> GASDSPMAYTDGSYQFILNADNTATITKYTGNEHRITIPAQVTHGAYIYPVSKIGDRVFCNYKYVLTSVQIPDTVTEIGSNAFYNCTSLKRVTIQDNKPSCVKKIGRQAFMFCSELTDIPILDSVTEIDSEAFHHCEELDTVTIPEGVTSVADGMFSYCYSLHTVTLPDSVTAIEERAFTGTALTQIHIPAKVTRIGTNAFSECFALSTITSDSESYPAIDNVLYEKSANGDYALIRYPSQREDPAFKIPNGVARIETHAFDSCAYLASVKMPDSVVSIGTGAFMNCPALQDIEFSSRITELPESVFAGCISL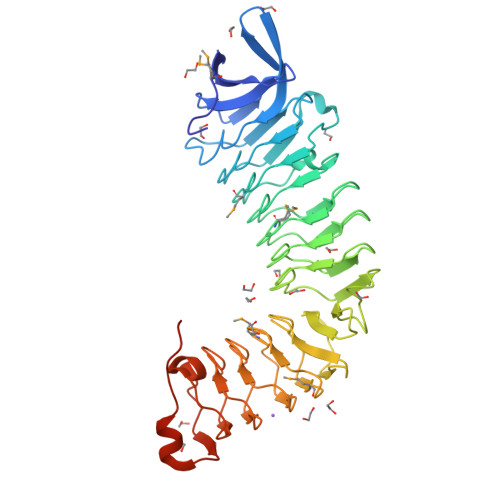KSIDIPEGITQILDDAFAGCEQLERIAIPSSVTKIPESAFSNCTALNNIEYSGSRSQWNAISTDSGLQNLPVAPGSIDVTV>[10x]APQNITELCSEYHNTQIYTINDKILS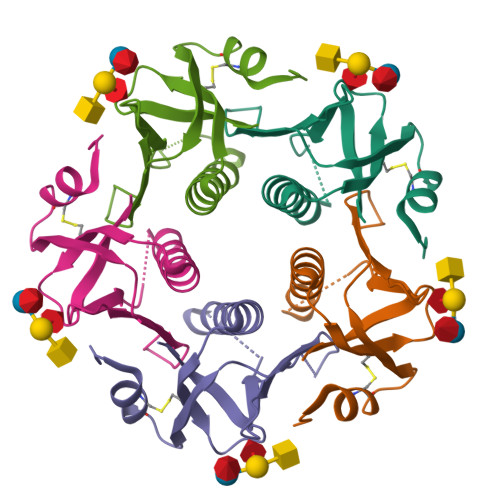YTESLAGKREMAIITFKNGATFQVEVPGSQHIDSQKKAIERMKDTLRIAYLTEAKVEKLCVWNNKTPNSIAAISMAN> MGLLLPLALCILVLCCGAMSPPQLALNPSALLSRGCNDSDVLAVAGFALRDINKDRKDGYVLRLNRVNDAQEYRRGGLGSLFYLTLDVLETDCHVLRKKAWQDCGMRIFFES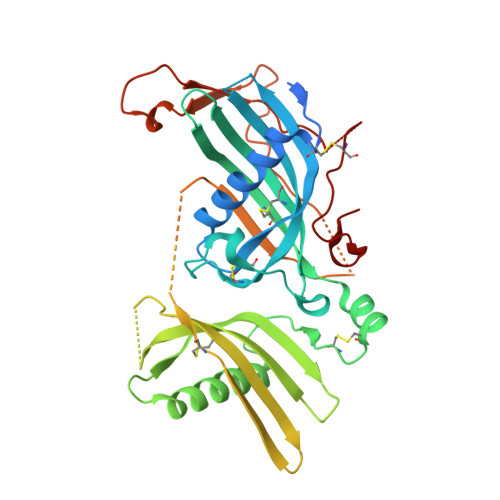VYGQCKAIFYMNNPSRVLYLAAYNCTLRPVSKKKIYMTCPDCPSSIPTDSSNHQVLEAATESLAKYNNENTSKQYSLFKVTRASSQWVVGPSYFVEYLIKESPCTKSQASSCSLQSSDSVPVGLCKGSLTRTHWEKFVSVTCDFFESQAPATGSENSAVNQKPTNLPKVEESQQKNTPPTDSPSKAGPRGSVQYLPDLDDKNSQEKGPQEAFPVHLDLTTNPQGETLDISFLFLEPMEEKLVVLPFPKEKARTAECPGPAQNASPLVLPPHHHHHH L-ALA-GAMMA-D-GLU-MESO-DIAMINOPIMELIC ACID 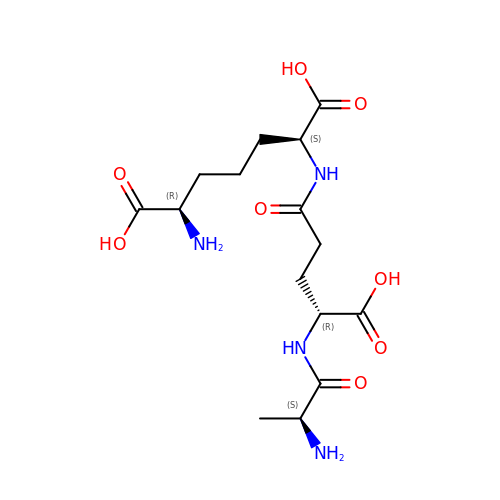| C15 H26 N4 O8 | FMNCPUGORYYCEM-QCLAVDOMSA-N>[2x]GSHMQNTFLDTIATRFDGTHSNFVLGNAQANGNPIVYCSDGFVDLTGYSRAQIMQKGCSCHFLYGPDTKEEHKQQIEKSLSNKMELKLEVIFYKKEGAPFWCLFDIVPIKNEKRDVVLFLASHKDITHTK

The KCNH family of voltage gated potassium channels includes the EAG (ether-a-go-go) channels, the ERG (eag related gene) channels and the ELK (eag like K+) channels; these channels have roles in cardiac repolarization, neuronal excitability, cell differentiation and tumor growth. A defining characteristic of KCNH channels is their large N- and C-terminal cytoplasmic regions. The N-terminus typically includes a Per-Arnt-Sim (PAS) domain, while the C-terminal region includes a domain that strongly resembles cyclic nucleotide binding domains, but which has been shown to have little affinity for cyclic nucleotides. As already stated, the role of PAS domains in KCNH channels is unknown; it is not known if these domains bind small ligands or mediate interactions between the channel and other proteins.

Crystals of dELK PAS domain were obtained after applying a strategy that involves methylation of lysines and removal of the first 10 amino acids of the protein. In the dELK PAS domain crystals, the asymmetric unit contains two very similar copies (rmsd 0.4 Å for main chain atoms of all residues). Analysis of the two dELK structures in the asymmetric unit reveals the absence of a large cavity. The lack of a preformed cavity in the dELK domain, at the same site as in hERG, appears to result from the presence of several large side-chains in that region. A large part of the volume is occupied by the side-chain of F110 in dELK, which substitutes the smaller valine residue present in hERG (V110). In dELK a histidine (H129) replaces the cavity lining phenylalanine present in hERG (F129). The absence of a cavity in dELK leaves the histidine side-chain buried in the domain hydrophobic core surrounded, within 5 Å, by the side-chains of several apolar residues (V30, F48, L51, L69,F98, F110 and A127) and two cysteines (C66 and C108). In contrast, in dELK the hydrophobic patch is not involved in crystal lattice packing. Instead part of the domain N-terminus forms an amphipathic α-helix (residues 14 to 21) which packs its apolar face against the hydrophobic patch on the surface of the β-sheet. Interestingly, a superposition of the dELK structure with the Δ9-hERG PAS domain through residues in their β-sheet reveals that the N-terminal helices occupy the same relative positions at the center of the hydrophobic patch of each domain.> GAMKLAELTLESDDFITSDKLFNFCKSTIFGAKYVKTDFIKFRQYQYIVSNCGWRDDTDVVFLENTPVLVTGHSDYDISEREIDIIRLPNIRAWFCQNRNIPHPKVISFPLGITNKDEPNSEIHRIIGNTDRILEVSKTPKEIKNLVYMNITVKNFPEERQRIVDLYSDKSWVTIGKGEVSEEGHRKFLEDMYAHKFCFAPRGNGIDTHRLWESLYLRTIPIVKKHIAMEQFTDLPILFVNDWENITEEYLNEQYDIIMAKDWNLDKLKIDYWYQKILEYSQ

Protein A075L is a β‐xylosyltransferase that participates in producing the core of the N‐glycans found in VP54, the major viral capsid protein of Paramecium bursaria chlorella virus‐1 (PBCV‐1). The protein structure shows a typical GT‐B folding, with two Rossmann‐like fold domains, in which the acceptor substrate binds to the N‐terminal region, and the nucleotide‐sugar donor binds to the C‐terminal region. We propose that the catalytic mechanism follows a direct displacement SN2‐like reaction, where Asp73 serves as a catalytic base that deprotonates the incoming nucleophile of the acceptor, facilitating direct displacement of the UDP with the inversion of the anomeric configuration of the acceptor without metal ion dependence, while the interactions with side chains of Arg158 and Arg208 stabilize the developing negative charge. In this context, we herein present the structural and biochemical characterization of A075L, a soluble chlorovirus xylosyltransferase easily produced in E. coli and amenable to large‐scale purification.

The crystal structure of A075L in complex with trisaccharide 6 shows a clear density map for the acceptor, including the octyl group. The Rha moiety is located within a deep pocket and establishes hydrogen bonds with His122 and Thr112. The Gal ring engages in four hydrogen bonds with residues Asn202, Ser72, Asp36, and Lys34, and is also somewhat exposed to the solvent. Given its close proximity to the acceptor, Asp73 appears to be the best‐positioned residue to act as a catalytic base, facilitating the deprotonation of Fuc O4. Analysis of the X‐Ray crystallographic structure of A075L bound to the trisaccharide provides an explanation for the observed specificity. The D‐Rha moiety is deeply inserted in the enzyme pocket, which, in turn, places the C4 hydroxyl group of the L‐Fuc moiety near Asp73. Deprotonation of this hydroxyl group by Asp73 facilitates nucleophilic attack on the donor. This exquisite arrangement highlights the specificity of the enzyme for a minimal acceptor motif. Epitope mapping analysis for the three acceptor substrates revealed that, despite minor differences in intensity, most of the protons of the three model acceptors showed up in all three STD NMR spectra. These results strongly suggest the existence of a groove‐type binding mode, wherein the entire ligand, particularly the Rha and Gal units, are embedded within the enzyme's binding site, rather than interacting with a shallow region. Thus, it appears that the motif present in 4 (α‐D‐Rha‐(1 → 3)‐α‐L‐Fuc), is the minimum acceptor for the enzyme.> SPSVEACGYSDRVAQLTVGNSTITTQEAANIVLSYGEWP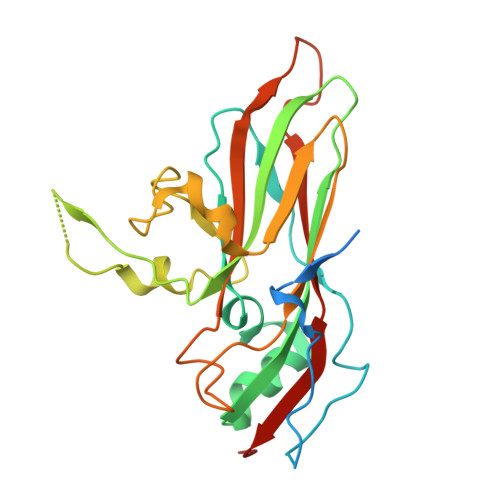EYCPSTDATAVDKPTRPDVSVNRFYTLSTKSWKTESTGWYWKFPDVLNDTGVFGQNAQFHYLYRSGFCMHVQCNASKFHQGALLVAAIPEFVIAASSPATKPNSQGLYPDFAHTNPGKDGQEFRDPYVLDAGIPLSQALIFPHQWINLRTNNCATIIMPYINALPFDSALNHSNFGLVVIPISPLKYCNGATTEVPITLTIAPLNSEFSGLRQAIKQ> MSWQTYVDEHLMCDIDGQGEELAASAIVGHDGSVWAQSSSFPQFKPQEITGIMKDFEEPGHLAPTGLHLGGIKYMVIQGEAGAV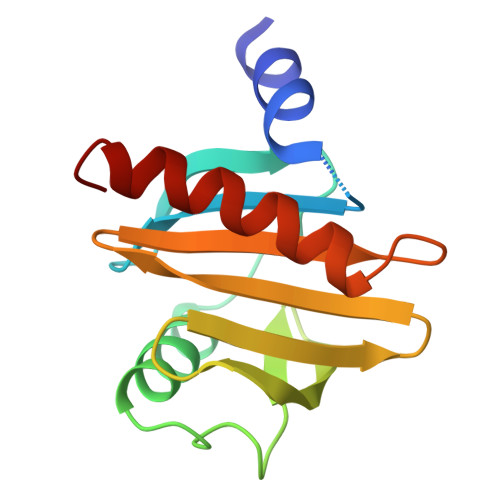IRGKKGSGGITIKKTGQALVFGIYEEPVTPGQCNMVVERLGDYLIDQGL>GPTEEQAAENWRDAMKTELQTIRTEIQEETARR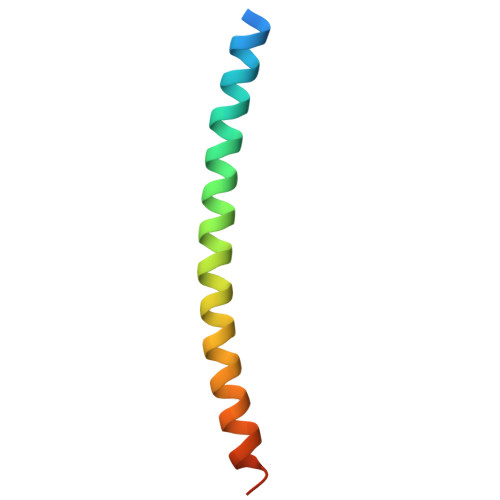QEELNAQNLVKMQELMSNFFQKITI[8x]As a zinc ion–dependent enzyme, CDA participates in the pyrimidine salvage pathway by converting cytidine and deoxycytidine into uridine and deoxyuridine. Bacteria extensively exhibit two forms of CDA: a long form and a short one. The former harbors two tandem CDA domains typically structured in a dimer assembly (homodimeric CDA or D-CDA), while the latter possesses a single catalytic domain arranged in a tetramer assembly (termed homotetrameric CDA or T-CDA). The CDA derived from E. faecium (EfCDA) belongs to the T-CDA form. EfCDA showed the ability to convert gemcitabine to its metabolite 2′,2′-difluorodeoxyuridine.

The full-length EfCDA protein, encompassing a singular CDA catalytic domain consisting of 132 amino acids, was purified. The structural architecture of EfCDA is composed of a five-stranded β-sheet (β1-β5) encircled by three α-helices (α1-α3). Moreover, the protein encompasses two elongated loops that function to connect α1 and β1 (loop 1), as well as β2 and α2 (loop 2), respectively. A zinc-dependent characteristic is exhibited by EfCDA, wherein the crystal structure revealed that a zinc ion was coordinated by three cysteine amino acids (C55, C88, and C91) and a water molecule. By previously elucidated crystal structures of CDAs from bacteria and yeast, the crystal structure of EfCDA also manifested the formation of a tetrameric assembly. Molecules A and B were in one asymmetric unit with an r.m.s.d. of 0.125 Å, and the complete tetramer was obtained through a symmetry-related operation. The interface area observed between molecules A and B was 1224.8 Å2, while molecules A and D measured 943.2 Å2, indicating a stable tetramer. The tetrameric structure of EfCDA is assembled through intermolecular interactions among specific residues in disparate subunits, particularly the α2-α2 and α3-α3 regions of neighboring molecules. Consequently, the enzyme's active site is encircled by specific residues, including Y23 from loop 1 on molecule C, A48 and F50 from loop 2 of molecule C, and F127 and L132 from the C-terminal loop of molecule D, which may facilitate the regulation of substrate and product ingress and egress.

>[2x]GSMAELKQEWINTAIEALDKAYVPYSHFPVGACLVTESGKIYQGINIENASFGLTNCAERTAFFKAVSEGERSFTHLVVAGHTPDPISPCGACRQVMAEFCAPDMPVTLVGDNGVTKATTVRELLPYAFTEKDL4-[[(1R)-2-[5-(2-fluoranyl-3-methoxy-phenyl)-3-[[2-fluoranyl-6-(trifluoromethyl)phenyl]methyl]-4-methyl-2,6-bis(oxidanylidene)pyrimidin-1-yl]-1-phenyl-ethyl]amino]butanoic 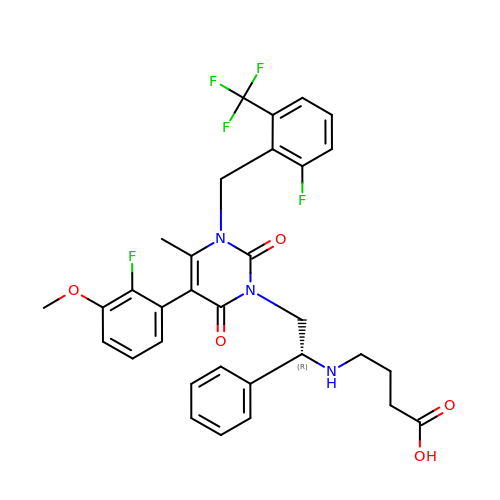acid | C32 H30 F5 N3 O5 | HEAUOKZIVMZVQL-VWLOTQADSA-N3,4-dihydro-2H-1,5-benzodioxepin-6-ylmethanamine | C10 H13 N O2 | 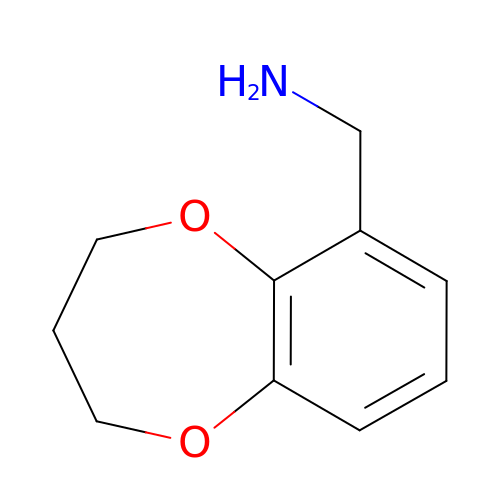ZXJOKQNPRXXPJT-UHFFFAOYSA-N>[2x]GPLGAAGLGHPAAFGRATHAVVRALPESLGQHALRSAKGEEVDVARAERQHQLYVGVLGSKLGLQVVELPADESLPDCVFVEDVAVVCEETALITRPGAPSRRKEVDMMKEALEKLQLNIVEMKDENATLDGGDVLFTGREFFVGLSKRTNQRGAE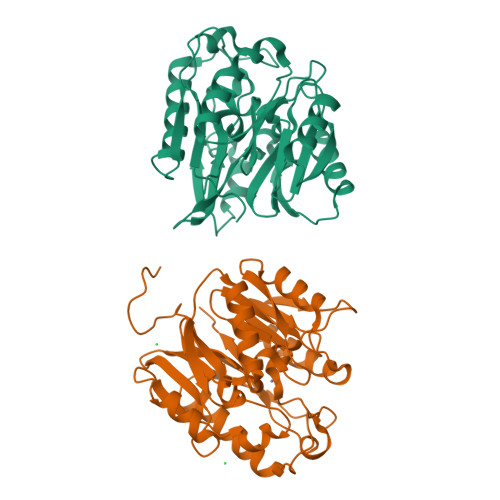ILADTFKDYAVSTVPVADGLHLKSFCSMAGPNLIAIGSSESAQKALKIMQQMSDHRYDKLTVPDDIAANCIYLNIPNKGHVLLHRTPEEYPESAKVYEKLKDHMLIPVSMSELEKVDGLLTCCSVLINKKVDS>MNKPVKKQQPKKVIPNF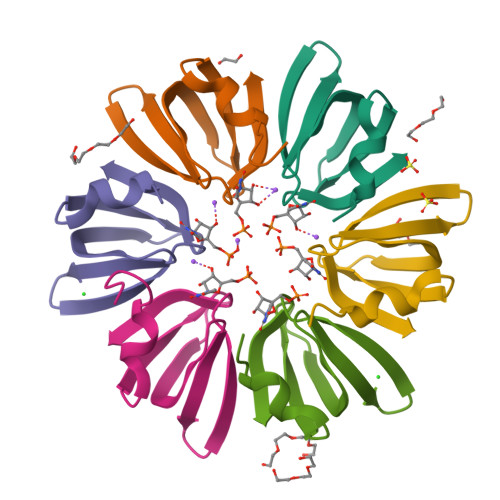EYARRLNGKKVKIFLRNGEVLDAEVTGVSNYEIMVKVGDRNLLVFKHAIDYIEY[6x]>[2x]SNADGLEGMDDPDATSKKVVPLGVEIYEINGPFFFGVADRLKGVLDVIEETPKVFILRMRRVPVIDATGMHALWEFQESCEKRGTILLLS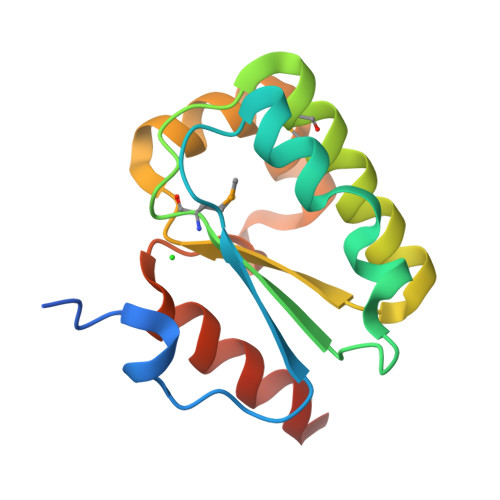GVSDRLYGALNRFGFIEALGEERVFDHIDKALAYAKLLVETAEER> GKECEFAMRLVPGFNPLRQVDANGKECRGNVELPFCKGYCKTSESGTHGFPPRVQNSK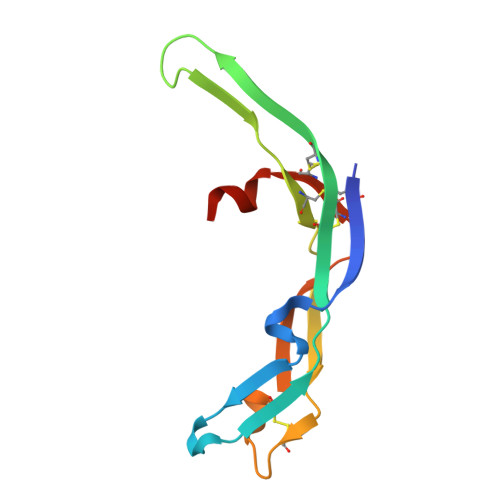VCTLVTTSTRKVVLDDCDDGADESVKFVMVPHGTDCECSAVPLEQHHS>[5x]MIGVNRMTEASTYIGTVQDVNGANIRVVLDINTISSLKFVDGQGYRIGQIGSFVRIPIGYINLFGIVSQVGAGAVPDKLLEVEPYGHRWISVQLVGEEGIKKEFERGVSQYPTIGDKVHIVTEPDLKKIYGTQNKKYISLGNIASVDSIPALVNIDTLVTRHSAVLGSTGSGKSTTVTSILQRISDMSQFPSARIIVFDIHGEYAAAFKGKAKVYKVTPSNNELKLSIPYWALTCDEFLSVAFGGLEGSGRNALIDKIYELKLQTLKRQEYEGINEDSLTVDTPIPFSIHKLWFDLYRAEISTHYVQGSHSEENEALLLGEDGNPVQKGDSLKVVPPIYMPHTQAQGATKIYLSNRGKNIRKPLEGLASLLKDPRYEFLFNADDWSVNLDGKTNKDLDALLETWVGSEESISIFDLSGMPSSILDTLIGILIRILYDSLFWSRNQPEGGRERPLLVVLEEAHTYLGKDSRGIAIDGVRKIVKEGRKYGIGMMLVSQRPSEIDSTILSQCGTLFALRMNNSSDRNHVLGAVSDSFEGLMGMLPTLRTGEAIIIGESVRLPMRTIISPPPFGRR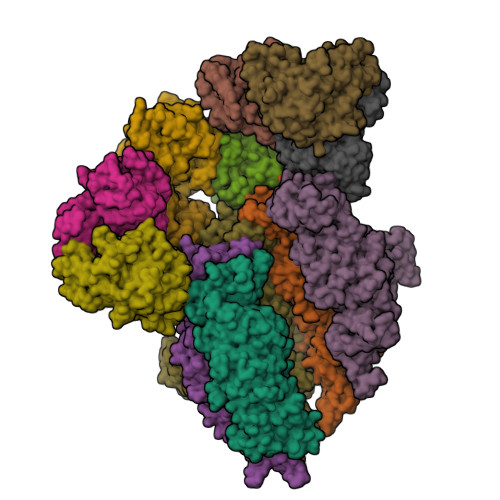PDSLDPDVTAKWSNNRVQGDYKEVLTLWRQKKVRSQRIVENIKRLPVVNEGEMTDMVREMVTSSNILSIGYEADSMTLEIEFNHGLVYQYYDVPETLHTELLAAESHGKFFNSQIKNNYRFSRI;>[8x]MDHSITASYYDTTQQLSLLKHVLSEDKRPIAFIIAAGCPVSIRHNDAPLIPDVAGLTRKISDSFGGNPDSLLMKIIQNLKTTIPNPTIEDILSYIRLLQQIPMSGKIHDVENSVINALEESICELIEEEVNVDLPGNATPYHKIAAWINSINREHQVEIFTTNYDLLMEQALEELNVPYFDGFVGSKRAFFDIRTIEENKLPSRWSKLWKLHGSINWQLDKQTQTIWRGTPSKGCSLIHPSHLKYDQSRKMPYLVMMDQLKLFLNQPSAILITCGYSYKDQHINEVLSQGLQTNPNALIYGLQYDVLENYQEAKDMALKRSNLILLAKDRAIIGKKEGEWKPDPQSSQDNDPLLFFKLGDFQHLASFLEEISQYDWSKQND>MDYKDDDDKMAGKRENFVRVDDLDSRLPSSSVAFQQNYASNFSGQLHPIHASNETSRSFKKGIQKGSKGLKSIGRSLGFGVYRAVFPEDLKVSEKKIFDPQDKFLLYCNKLFVASCILSVFVDPFFFYLPVINAESKCLGIDRKLAITASTLRTFIDVFYLAHMALQLRTAYIAPSSRVFGRGELVIDPAQIAKRYLQRWFIIDFLSVLPLPQIVVWRFLQSSNGSDVLATKQALLFIVLVQYIPRFLRVLPLTSELKRTAGVFAETAWAGAAYYLLLYMLASHIVGAFWYLLALERNDACWQEACIDAGNCSTDFLYCGNQNMDGYAVWNRAKESVLKSKCRADLDDNNPPFDFGIYTQALSSGIVSSQNFIVKYCYCLWWGLQNLSTLGQGLETSTYPMEIIFSISLAISGLILFALLIGNMQTYLQ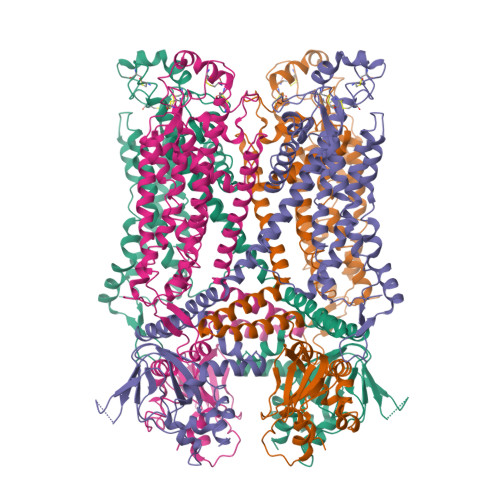SLTIRLEEMRVKRRDSEQWMHHRMLPQDLRERVRRYDQYKWLETRGVDEEYLVQNLPKDLRRDIKRHLCLALVRRVPLFKSMDDKLLDAICMRLKPCLFTESTYLVREGDPVDEMLFIIRGRLESVTTDGGRSGFFNRSLLKEGEFCGEELLTWALDPKSGVNLPSSTRTVKALTEVEAFALTSEELKFVASQFRRLHSRQVQHTFRFYSHQWRTWAACFIQAAWRRYCKRKKMEEAEAEAAAVSSSTAGPSYSIGAAFLATKFAANALRTIHRNRNTKIRDLVKLQKPPEPDFTAD[4x]> EDQVDPRLIDGKGRTCPKPDDLPFSTVVPLKTFYEPGEEITYSCKPGYVSRGGMRKFICPLTGLWPINTLKCTPRVCPFAGILENGAVRYTTFEYPNTISFSCNTGFYLNGADSAKCTEEGKWSPELPVCAPIICPPPSIPTFATLRVYKPSAGNNSLYRDTAVFECLPQHAMFGNDTITCTTHGNWTKLPECREVKCPFPSRPDNGFVNYPAKPTLYYKDKATFGCHDGYSLDGPEEIECTKLGNWSAMPSCKASCKVPVKKATVVYQGERV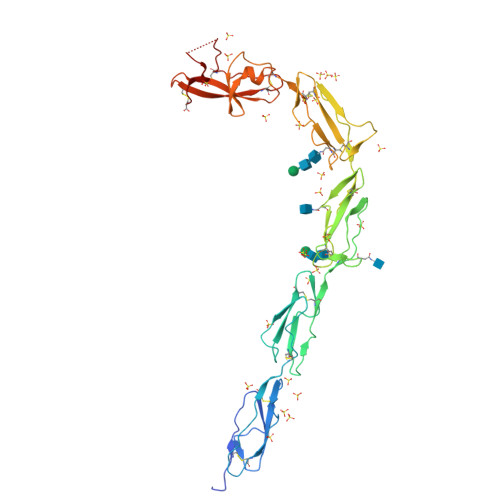KIQEKFKNGMLHGDKVSFFCKNKEKKCSYTEDAQCIDGTIEVPKCFKEHSSLAFWKTDASDVKPC>[3x]MRPVYFLSDFGLEDPYVAVVKAVLAERAPGPAVVDLAHALPPQDLRRAAYALFEALPYLPEGAVVLAVVDPGVGTARRAVAALGRWTYVGPDNGLFTLAWLLDPPRRAFLLEPPRPRPKAALPGWAPGEATFHGRDVFAPAAAHLALGLPPEGLGPEVPVETLARLPLALTEGPEGEVLTFDRFGNAITTLLRAPVGGFVEVGGRRVPVRRTFGEVPEGAPVAYLGSAGLLEVAVNRGSAREALGLKEGM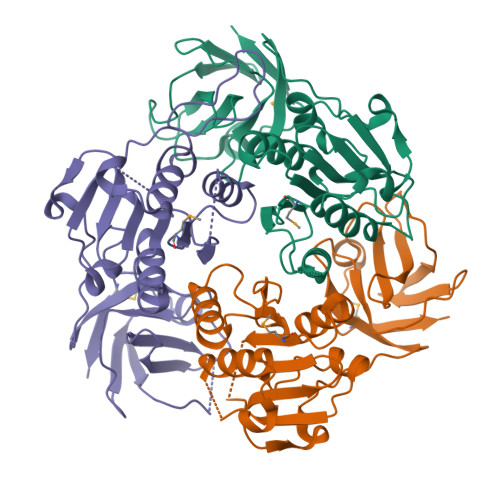PVRLL>MANLKENIVWEHVFDNCSQANVVFSY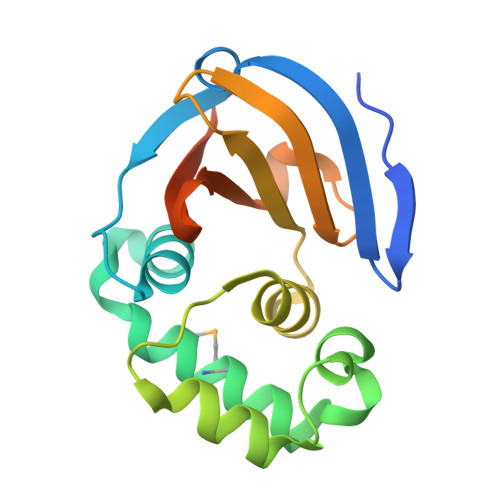REFFNKELTLPDGNCFFRAVSTFLYDTQNGWIEVKNMCREFAETNWDELPGVHQYFQDPEHYARESKREGYWGGSVEAEILSKLLKLTVIFWKCEDDVWVTQGIRWGDGNYLTAINLLHIQFDHFDFLVPINVTQEPPKSGSHHHHHH[3x]>MKMVVAVIRPEKLECVKKALEERGFVGMTVTEVKGRGEQKGIRLQFRGREVEVDLLQKTKVEVVVSDDAVDEVVEAIVSSARTGKFGDG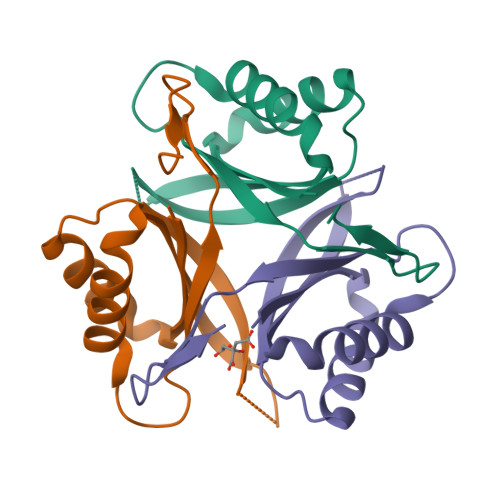RIFVIPVEKSVKIRTGDEEVAAAHHHHHH[6x]> MGVFRTRFTETFGVEHPIMQGGMQWVGRAEMAAAVANAGGLATLSA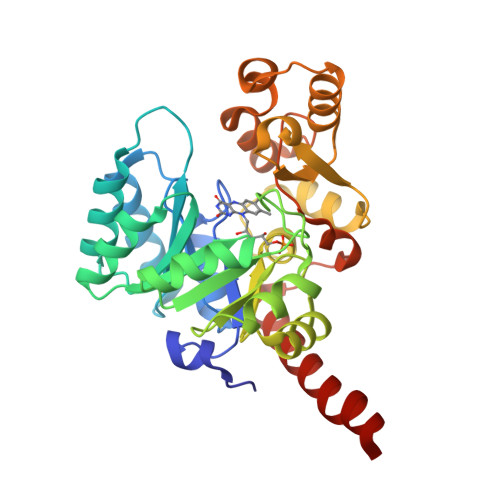LTQPSPEALAAEIARCRELTDRPFGVNLTLLPTQKPVPYAEYRAAIIEAGIRVVETAGNDPGEHIAEFRRHGVKVIHKCTAVRHALKAERLGVDAVSIDGFECAGHPGEDDIPGLVLLPAAANRLRVPIIASGGFADGRGLVAALALGADAINMGTRFLATRECPIHPAVKAAIRAADERSTDLIMRSLRNTARVARNAISQEVLAIEARGGAGYADIAALVSGQRGRQVYQQGDTDLGIWSAGMVQGLIDDEPACAELLRDIVEQARQLVRQRLEGMLAGV> MQSTITSTTSLTPQQILNQIIKPEYIKYYSDWIHTANEKEARGLQLLGAIYKHKGSKKFRAKPPSVQLQQLHAQQEFDFQKA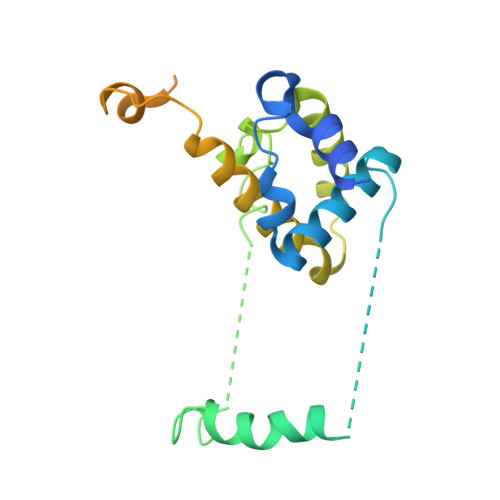EEMYRKSQITSSYGQEFGYLQKDLKPTQNVFKYKKCSDLPFAKPLSDLAKLFIDNWIELNDELEFQELVLACLRSLHSRCIAQEVPKTEMKTKYEWKEDWNLSKPIRIDKAGSDLKAYKTNYNAIFKQRLKQEHINEQLKQLDNSDFAKQLKIFKPFKIN> MEGLLFPVLSLGGLGVVFGLLLGYASKKFAVEVDERVPMVRAALPGANCGGCGFAGCDAYADAVVNAGAKPNGCPVG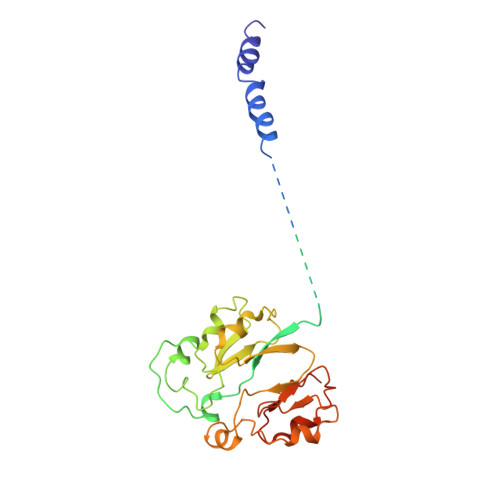GAACAAKIAEIMGVVVDSSEPKKAYVKCQGTCDKAKEKYEYYGAMTCVDAANIPGAGSKTCGFGCLGLGSCVQVCAFDAIHVENGIAVVDEEACTGCGACVSICPKSVIELTPMSKKVRISCNSHDKGIEVKNACSVGCLSCGLCVRNCPSEAITMVNNLPVIDYDKCTQCGVCVGKCPTKAIVNLNTNVSKEASNN> PITINNFRYSDPVNNDTIIMMEPPYCKGLDIYYKAFKITDRIWIVPERYEFGTKPEDFNPPSSLIEGASEYYDPNYLRTDSDKDRFLQTMVKLFNRIKNNVAGEALLDKIINAIPYLGNSYSLLDKFDTNSNSVSFNLLEQDPSGATTKSAMLTNLIIFGPGPVLNKNEVRGIVLRVDNKNYFPCRDG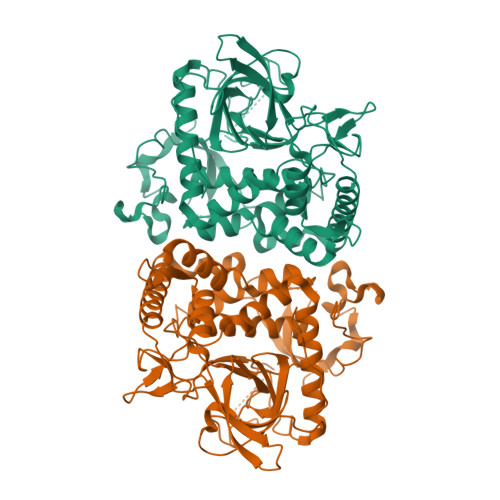FGSIMQMAFCPEYVPTFDNVIENITSLTIGKSKYFQDPALLLMHELIHVLHGLYGMQVSSHEIIPSKQEIYMQHTYPISAEELFTFGGQDANLISIDIKNDLYEKTLNDYKAIANKLSQVTSCNDPNIDIDSYKQIYQQKYQFDKDSNGQYIVNEDKFQILYNSIMYGFTEIELGKKFNIKTRLSYFSMNHDPVKIPNLLDDTIYNDTEGFNIESKDLKSEYKGQNMRVNTNAFRNVDGSGLVSKLIGLCKKIIPPTNIRENLYNRTASPPTPGHHHHHH> MADTQYILPNDIGVSSLDSREAFRLLSPTERLYAYHLSRAAWYGGLAVLLQTSPEAPYIYALLSRLFRAQDPDQLRQHALAEGLTEEEYQAFLVYAAGVYSNMGNYKSFGDTKFVPNLPKEKLERVILGSEAAQQHPEEVRGLWQTCGELMFSLEPRLRHLGLGKEGITTYFSGNCTMEDAKLAQDFLDSQNLSAYNTRLFKEVDGCGKPYYEVRLASVLGSEPSLDSEVTSKLKSYEFRGSPFQVTRGDYAPILQKVVEQLEKAKAYAANSHQGQMLAQYIESFTQGSIEAHKRGSRFWIQDKGPIVESYIGFIESYRDPFGSRGEFEGFVAVVNKAMSAKFERLVASAEQLLKELPWPPTFEKDKFLTPDFTSLDVLTFAGSGIPAGINIPNYDDLRQTEGFKNVSLGNVLAVAYATQREKLTFLEEDDKDLYILWKGPSFDVQVGLHALLGHGSGKLFVQDEKGAFNFDQETVINPETGEQIQSWYRCGETWDSKFSTIASSYEECRAESVGLYLSLHPQVLEIFGFEGADAEDVIYVNWLNMVRAGLLALEFYTPEAFNWRQAHMQARFVILRVLLEAGEGLVTITPTTGSDGRPDARVRLDRSKIRSVGKPALERFLRRLQVLKSTGDVAGGRALYEGYATVTDAPPESFLTLRDTVLLRKESRKLIVQPNTRLEGSDVQLLEYEASAAGLIRSFSERFPEDGPELEEILTQLATADARFW;> IVYPW

Human dipeptidyl peptidase III (hDPP III), also known as enkephalinase B, is a member of the M49 family of zinc dependent metallopeptidases and cleaves dipeptides sequentially from the N-terminus of various bioactive peptide substrates. Crystal structures have so far been determined for DPP III from humans as well as from Saccharomyces cerevisiae. Despite the low sequence identity (36%) shared by the two proteins, both structures are very similar and consist of two lobes separated by a wide cleft. The “upper” lobe is mostly α-helical and contains the zinc binding site as well as the catalytically important residues. In both structures, two histidine residues (His-450 and His-455 in the human enzyme) and a glutamate (Glu-508) coordinate the zinc ion.

Similar to tynorphin (VVYPW), which is a derivative of spinorphin29 and has been shown to inhibit partially purified DPP III from monkey brain22, IVYPW inhibited rat DPP III with nanomolar affinity. IVYPW was in fact found to be a stronger inhibitor than tynorphin. In the present structure, IVYPW binds in the same mode as VVYPW and the other peptides discussed so far including the formation of the antiparallel β-strand interaction and the hydrogen bond from His-568. In addition, the zinc ion is coordinated by the carbonyl oxygen of Val-2 similar as in the complex with endomorphin-2. When analysing the interactions with the catalytic zinc ion, we observed that the carbonyl group of the scissile peptide bond is not directly interacting with the catalytic zinc ion (3.7 Å distance) in the complexes with Met- and Leu-enkephalin and a water molecule is bound to the ion. Instead, the metal ion is coordinated by the respective carbonyl group in the complex with the inhibitory IVYPW and there is no room for an additional water molecule. In the inhibitor (IVYPW) complex, on the other hand, the water molecule is missing. The modelled side chain of Glu-451 is about 4 Å from the scissile peptide bond and thus could directly act as the nucleophile leading to the formation of an acyl-enzyme-like intermediate. Based on the similarity between CPA and hDPP III, we hypothesize that inhibitory peptides, such as IVYPW and tynorphin, might displace the water molecule originally bound to the zinc ion. In this case the reaction may still follow the energetically unfavourable and therefore slow anhydride pathway.> KPGDIFEVELAKNDNSLGISVTGGVNTSVRHGGIYVKAVIPQGAAESDGRIHKG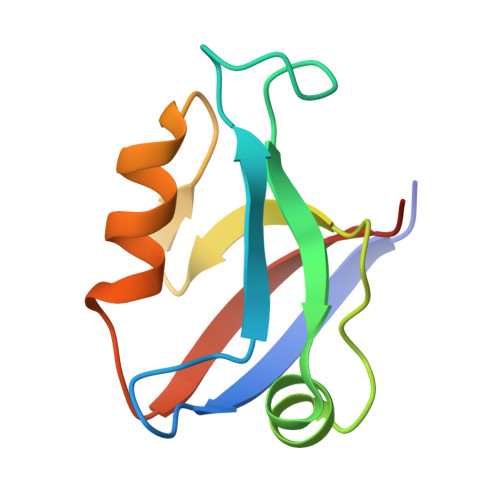DRVLAVNGVSLEGATHKQAVETLRNTGQVVHLLLEKGQSPT The L-tryptophan biosynthesis regulator, TRAP, present in several Bacilli, is a good model system for investigating determinants of the oligomeric state. The tryptophan RNA-binding attenuation protein, TRAP, possesses similar geometric features to other circular assemblies, being assembled of multiple subunits and containing a central tunnel. When activated by increased levels of L-tryptophan – bound to receptor sites nestled between adjacent subunits – TRAP binds single stranded RNA at the leader region of the trpEDCFBA operon transcript. This modulates terminator hairpin formation and so downregulates L-tryptophan biosynthesis.

A short segment of C-terminal residues defines whether TRAP forms an 11-mer or 12-mer assembly. However, this work required deletion of the C-terminus to increase the subunit stoichiometry and we questioned if a more subtle mutation at the C-terminus could induce formation of a 12-subunit assembly. Based on the previous structural work, we chose the S72N mutation because we expected that the bulky side chain at this position would result in the exclusion of N72 and following C-terminal residues from the subunit interface. Finally, we show how the 11-subunit to 12-subunit switch could be induced by the point mutation S72N. From the structure of the S72N TRAP we see that substituting serine 72 for a bulkier amino acid, asparagine, does indeed introduce the necessary constraints to exclude the subsequent segment from the subunit interface. Exclusion of the C-terminus from the subunit interface can be achieved by introducing steric strain at a key region towards the C-terminus that causes the segment to pivot out. In this respect, exclusion of the C-terminus in S72N is achieved in a manner more similar to how exclusion is achieved in B. halodurans TRAP. To understand if the 12-mer state of the S72N TRAP observed in the X-ray structure, predominates in solution, we analyzed this protein by native mass spectrometry. The 12-mer state was identified as the dominant species in the mass spectra, as opposed to the wild type protein which forms 11-mers. For instance, we note that both B. subtilis and B. stearothermophilus wild type TRAP contain two flexible lysine residues at their C-termini that can contribute electrostatically to the overall stability of TRAP. To understand which of these two factors – C-terminus or oligomeric state – has the greater influence we compared thermal stability of wild type B. subtilis TRAP 11-mer with that of the B. subtilis S72N TRAP 12-mer, which still possesses the C-terminal segment but has it excluded from the subunit interface for steric reasons.

>MNQKHSSDFVVIKAVEDGVNVIGLTRGTDTKFHHSEKLDKGEVIIAQFTEHTSAIKVRGEALIQTAYGEMKNEKK[6x]> SSLDDKPQFPGASAEFIDKLEFIQPNVISGIPIYRVMDRQGQIINPSEDPHLPKEKVLKLYKSMTLLNTMDRILYESQRQG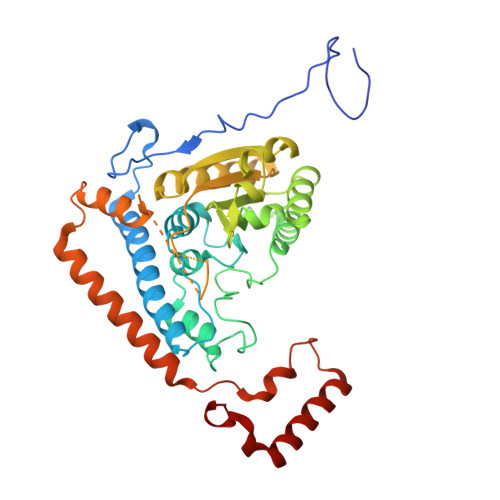RISFYMTNYGEEGTHVGSAAALDNTDLVFGAAREAGVLMYRDYPLELFMAQCYGNISDLGKGRQMPVHYGCKERHFVTISSPLATQIPQAVGAAYAAKRANANRVVICYFGEGAASEGDAHAGFNFAATLECPIIFFCRNNGYAISTPTSEQYRGDGIAARGPGYGIMSIRVDGNDVFAVYNATKEARRRAVAENQPFLIEAMTYRIGHHSTSDDSSAFRSVDEVNYWDKQDHPISRLRHYLLSQGWWDEEQEKAWRKQSRRKVMEAFEQAERKPKPNPNLLFSDVYQEMPAQLRKQQESLARHLQTYGEHYPLDHFDK> MGSVNSSPNEEFETVPDSQISGFDSPLIPTSVGSYFRDDDDDEKVHPNFISDPENDSLNSDEEFSSLENSDLNLSGAKAESGDDFDPILKRTIISKRKAPSNNEDEEIVKTPRKLVNYVPLKIFNLGDSFDDTITTTVAKLQDLKKEILDSPRSNKSIVITSNTVAKSELQKSIKFSGSIPEIYLDVVTKETISDKYKDWHFISKNCHYEQLMDLEMKDTAYSFLFGSSRSQGKVPEFVHLKCPSITNLLVLFGVNQEKCNSLKINYEKKENSRYDNLCTIFPVNKMLKFLMYFYSDDDNDDVREFFLKAFICLILDRKVFNAMESDHRLCFKVLELFNEAHFINSYFEIVDKNDFFLHYRLLQIFPHLQSALLRRRFSEKQGRTETIQQNIIKEFNEFFDCKNYKNLLYFILTMYGSKFIPFGPKCQVTEYFKDCILDISNETTNDVEISILKGILNLFSKIR;> MDGALINSVLYVSPRNGAHYFVELTEKHLLAFEMLNSMCLLENYDHVLLFLECQFGKSHNLAVIPFDIILVLFTLSTLSEYYKEPILRANDPYNTSRETLSRRALKLLQKYLAILKEFDSEQYNLYDLELLRCQFFLAIDTLTPKKQKWGFDRFRRTKSESGVTYRQNASVDPELDQAKTFKNPYRSYISCLEQRNTILGNRLLNLKLNEPGEFINMILWTLSNSLQESTPLFLSSHEIWMPLLEILIDLFSCRQDYFIQHEVAQNVSKSLFVQRLSESPLAVFFESLNTRNFANRFSEYVFLNCDYKLPSDNYATPVHPVYNGENTIVDTYIPTIKCSPLYKSQKSLALRRKLIGSCFKLLLRVPDGHRLITPRIVADDVIQGISRTLASFNDILQFKKFFMTENLSQESYFIPLLAEGTLSEILKDTQECVVILTLVENLSDGVSFCNEVIGLVKSKCFAFTEQCSQASYEEAVLNIEKCDVCLLVLLRYLLHLIGTEAILDAKEQLEMLHAIEKNDSGRRQWAKALNLGNDPPLLYPIVSQMFGVHDKSVIIE;> MTSLIDLGRYVERTHHGEDTEPRSKRVKIAKPDLSSFQPGSIIKIRLQDFVTYTLTEFNLSPSLNMIIGPNGSGKSTFVCAVCLGLAGKPEYIGRSKKVEDFIKNGQDVSKIEITLKNSPNVTDIEYIDARDETIKITRIITRSKRRSDYLINDYQVSESVVKTLVAQLNIQLDNLCQFLSQERVEEFARLKSVKLLVETIRSIDASLLDVLDELRELQGNEQSLQKDLDFKKAKIVHLRQESDKLRKSVESLRDFQNKKGEIELHSQLLPYVKVKDHKEKLNIYKEEYERAKANLRAILKDKKPFANTKKTLENQVEELTEKCSLKTDEFLKAKEKINEIFEKLNTIRDEVIKKKNQNEYYRGRTKKLQATIISTKEDFLRSQEILAQTHLPEKSVFEDIDIKRKEIINKEGEIRDLISEIDAKANAINHEMRSIQRQAESKTKSLTTTDKIGILNQDQDLKEVRDAVLMVREHPEMKDKILEPPIMTVSAINAQFAAYLAQCVDYNTSKALTVVDSDSYKLFANPILDKFKVNLRELSSADTTPPVPAETVRDLGFEGYLSDFITGDKRVMKMLCQTSKIHTIPVSRRELTPAQIKKLITPRPNGKILFKRIIHGNRLVDIKQSAYGSKQVFPTDVSIKQTNFYQGSIMSNEQKIRIENEIINLKNEYNDRKSTLDALSNQKSGYRHELSELASKNDDINREAHQLNEIRKKYTMRKSTIETLREKLDQLKREARKDVSQKIKDIDDQIQQLLLKQRHLLSKMASSMKSLKNCQKELISTQILQFEAQNMDVSMNDVIGFFNEREADLKSQYEDKKKFVKEMRDTPEFQSWMREIRSYDQDTKEKLNKVAEKYEEEGNFNLSFVQDVLDKLESEIAMVNHDESAVTILDQVTAELRELEHTVPQQSKDLETIKAKLKEDHAVLEPKLDDIVSKISARFARLFNNVGSAGAVRLEKPKDYAEWKIEIMVKFRDNAPLKKLDSHTQSGGERAVSTVLYMIALQEFTSAPFRVVDQINQGMDSRNERIVHKAMVENACAENTSQYFLITPKLLTGLHYHEKMRIHCVMAGSWIPNPSEDPKMIHFGETSNYSFD;> MISTTISGKRPIEQVDDELLSLTAQQENEEQQQQRKRRRHQFAPMTQFNSNTLDEDSGFRSSSDVATADQDNFLEESPSGYIKKVILRNFMCHEHFELELGSRLNFIVGNNGSGKSAILTAITIGLGAKASETNRGSSLKDLIREGCYSAKIILHLDNSKYGAYQQGIFGNEIIVERIIKRDGPASFSLRSENGKEISNKKKDIQTVVDYFSVPVSNPMCFLSQDAARSFLTASTSQDKYSHFMKGTLLQEITENLLYASAIHDSAQENMALHLENLKSLKAEYEDAKKLLRELNQTSDLNERKMLLQAKSLWIDVAHNTDACKNLENEISGIQQKVDEVTEKIRNRQEKIERYTSDGTTIEAQIDAKVIYVNEKDSEHQNARELLRDVKSRFEKEKSNQAEAQSNIDQGRKKVDALNKTIAHLEEELTKEMGGDKDQMRQELEQLEKANEKLREVNNSLVVSLQDVKNEERDIQHERESELRTISRSIQNKKVELQNIAKGNDTFLMNFDRNMDRLLRTIEQRKNEFETPAIGPLGSLVTIRKGFEKWTRSIQRAISSSLNAFVVSNPKDNRLFRDIMRSCGIRSNIPIVTYCLSQFDYSKGRAHGNYPTIVDALEFSKPEIECLFVDLSRIERIVLIEDKNEARNFLQRNPVNVNMALSLRDRRSGFQLSGGYRLDTVTYQDKIRLKVNSSSDNGTQYLKDLIEQETKELQNIRDRYEEKLSEVRSRLKEIDGRLKSTKNEMRKTNFRMTELKMNVGKVVDTGILNSKINERKNQEQAIASYEAAKEELGLKIEQIAQEAQPIKEQYDSTKLALVEAQDELQQLKEDINSRQSKIQKYKDDTIYYEDKKKVYLENIKKIEVNVAALKEGIQRQIQNACAFCSKERIENVDLPDTQEEIKRELDKVSRMIQKAEKSLGLSQEEVIALFEKCRNKYKEGQKKYMEIDEALNRLHNSLKARDQNYKNAEKGTCFDADMDFRASLKVRKFSGNLSFIKDTKSLEIYILTTNDEKARNVDTLSGGEKSFSQMALLLATWKPMRSRIIALDQFDVFMDQVNRKIGTTLIVKKLKDIARTQTIIITPQDIGKIADIDSSGVSIHRMRDPERQNNSNFYN;> MSSTVISRKRRNSTVTEPDSSGETRKQKKSRSDEKSSSSKDGDPQLEFKVLQGYRDLESEMHKGRAQVTRTGDIGVAMDNLNAVDSLFNKVIGIKNNGLFAHDARAMVSISELAQISVRNLKFDDSRSMVNLENIVNSLKRYMLKEHFKLNNIAENRNDLTLAADEQ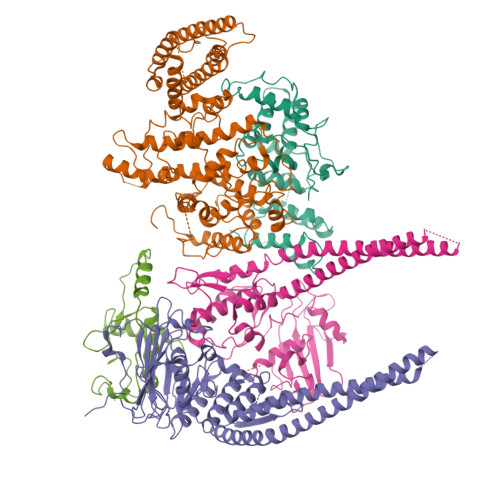SAADQQEESDGDIDRTPDDNHTDKATSSFKATSMRHSYLQQFSHYNEFSQFNWFRIGALYNTISKNAPITDHLMGPLSIEKKPRVLTQRRRNNDQVGEKITAEKITQHSLNSTQQETTPEQVKKCFKKLSKKLGPEGSINLFKFIIDPNSFSRSIENLFYTSFLIKEGKLLMEHDEEGLPTIKIKQSISHTDSRSKEIERQRRRAAHQNHIIFQMDMPTWRKLIKKYNITSPFLD> MAAPARDPPGYRYAAAMVPTGSILSTIEVASHRRLFDFFAAVRSDENSLYDVEFDALLGSYCNTLSLVRFLELGLSVACVCTKFPELAYMNEGRVQFEVHQPLIARDGPHPVEQPVHNYMTKVIDRRALNAAFSLATEAIALLTGEALDGTGISLHRQLRAIQQLARNVQAVLGAFERGTADQMLHVLLEKAPPLALLLPMQRYLDNGRLATRVARATLVAELKRSFCDTSFFLGKAGHRREAIEAWLVDLTTATQPSVAVPRLTHADTRGRPVDGVLVTTAAIKQRLLQSFLKVEDTEADVPVTYGEMVLNGANLVTALVMGKAVRSLDDVGRHLLDMQEEQLEANRETLDELESAPQTTRVRADLVAIGDRLVFLEALEKRIYAATNVPYPLVGAMDLTFVLPLGLFNPAMERFAAHAGDLVPAPGHPEPRAFPPRQLFFWGKDHQVLRLSMENAVGTVCHPSLMNIDAAVGGVNHDPVEAANPYGAYVAAPAGPGADMQQRFLNAWRQRLAHGRVRWVAECQMTAEQFMQPDNANLALELHPAFDFFAGVADVELPGGEVPPAGPGAIQATWRVVNGNLPLALCPVAFRDARGLELGVGRHAMAPATIAAVRGAFEDRSYPAVFYLLQAAIHGNEHVFCALARLVTQCITSYWNNT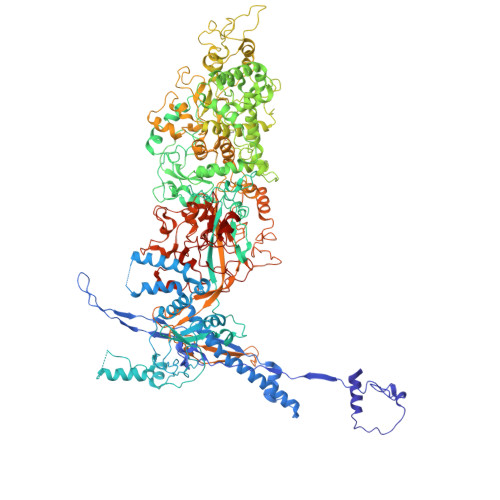RCAAFVNDYSLVSYIVTYLGGDLPEECMAVYRDLVAHVEALAQLVDDFTLPGPELGGQAQAELNHLMRDPALLPPLVWDCDGLMRHAALDRHRDCRIDAGGHEPVYAAACNVATADFNRNDGRLLHNTQARAADAADDRPHRPADWTVHHKIYYYVLVPAFSRGRCCTAGVRFDRVYATLQNMVVPEIAPGEECPSDPVTDPAHPLHPANLVANTVKRMFHNGRVVVDGPAMLTLQVLAHNMAERTTALLCSAAPDAGANTASTANMRIFDGALHAGVLLMAPQHLDHTIQNGEYFYVLPVHALFAGADHVANAPNFPPALRDLARHVPLVPPALGANYFSSIRQPVVQHARESAAGENALTYALMAGYFKMSPVALYHQLKTGLHPGFGFTVVRQDRFVTENVLFSERASEAYFLGQLQVARHETGGGVNFTLTQPRGNVDLGVGYTAVAATGTVRNPVTDMGNLPQNFYLGRGAPPLLDNAAAVYLRNAVVAGNRLGPAQPLPVFGCAQVPRRAGMDHGQDAVCEFIATPVATDINYFRRPCNPRGRAAGGVYAGDKEGDVIALMYDHGQSDPARPFAATANPWASQRFSYGDLLYNGAYHLNGASPVLSPCFKFFTAADITAKHRCLERLIVETGSAVSTATAASDVQFKRPPGCRELVEDPCGLFQEAYPITCASDPALLRSARDGEAHARETHFTQYLIYDASPLKGLSL> MAPLGYFLLLCSLKQALGSYPIWWSLAVGPQYSSLGSQPILCASIPGLVPKQLRFCRNYVEIMPSVAEGIKIGIQECQHQFRGRRWNCTTVHDSLAIFGPVLDKATRESAFVHAIASAGVAFAVTRSCAEGTAAICGCSSRHQGSPGKGWKWGGCSEDIEFGGMVSREFADARENRPDARSAMNRHNNEAGRQAIASHMHLKCKCHGLSGSCEVKTCWWSQPDFRAIGDFLKDKYDSASEMVVEKHRESRGWVETLRPRYTYFKVPTERDLVYYEASPNFCEPNPETGSFGTRDRTCNVSSHGIDGCDLLCCGRGHNARAERRREKCRCVFHWCCYVSCQECTRVYDVHTCK;> MAGAIIENMSTKKLCIVGGILLVFQIIAFLVGGLIAPGPTTAVSYMSVKCVDARKNHHKTKWFVPWGPNHCDKIRDIEEAIPREIEANDIVFSVHIPLPHMEMSPWFQFMLFILQLDIAFKLNNQIRENAEVSMDVSLAYRDDAFAEWTEMAHERVPRKLKCTFTSPKTPEHEGRYYECDVLPFMEIGSVAHKFYLLNIRLPVNEKKKINVGIGEIKDIRLVGIHQNGGFTKVWFAMKTFLTPSIFIIMVWYWRRITMMSRPPVLLEKVIFALGISMTFINIPVEWFSIGFDWTWMLLFGDIRQGIFYAMLLSFWIIFCGEHMMDQHERNHIAGYWKQVGPIAVGSFCLFIFDMCERGVQLTNPFYSIWTTDIGTELAMAFIIVAGICLCLYFLFLCFMVFQVFRNISGKQSSLPAMSKVRRLHYEGLIFRFKFLMLITLACAAMTVIFFIVSQVTEGHWKWGGVTVQVNSAFFTGIYGMWNLYVFALMFLYAPSHKNYGEDQSNGDLGVHSGEELQLTTTITHVDGPTEIYKLTRKEAQE

Wntless (WLS), an evolutionarily conserved multi-pass transmembrane protein, is essential for secretion of Wnt proteins. WLS has been found to directly interact with Wnts throughout the secretory route initiated from ER, then Golgi, secretory vesicles and finally cell membrane. Wnt-triggered signaling pathways control many crucial life events, whereas aberrant Wnt signaling is tightly associated with many human diseases including cancers. The transmembrane domain of WLS bears a GPCR fold, with a conserved core cavity and a lateral opening.

Here, we report a cryo-EM structure of wild type (WT) human WLS in complex with Wnt3a at 2.2 Å resolution. The built model comprises 496 residues of 541-residue WLS and 334 residues of Wnt3a after cleavage of signal peptide. In the overall structure, Wnt3a perches on the luminal side of WLS with several β-hairpin and loop regions (Hairpin-1, Hairpin-2 and W-loop) interacting with WLS extensively and generate three major interfaces. WLS looks like a grasping right hand that seizes one finger (Hairpin-1) of Wnt3a bearing the conserved palmitoleoylated Ser209, which is reported to be essential for Wnt secretion and interaction with Frizzled receptors on cell membrane. Wnt3a pinches WLS with another two fingers (Hairpin-2 and W-loop) at the luminal region of WLS. Wnt3a is palmitoleoylated with density for PAM clearly resolved, and the modification was confirmed by mass spectrometry. Intriguingly, we found in the TM domain of WLS there is a large hydrophobic cavity and a lateral opening between TM6 and TM7 that exposes the cavity to membrane environment. This cavity accommodates the extruding Hairpin-1 of Wnt3a, and one POPC molecule, clearly identified in the EM map. At Interface 2, Wnt3a Hairpin-2, containing Trp333 and stabilized by the disulfide bond formed between Cys334 and Cys335, extensively interacts with residues in a hydrophobic pocket at the distal region of WLS luminal domain. At Interface 3, Trp150 on Wnt3a W-loop forms hydrophobic interactions with Met101, Met103, and Phe107 in the loop between β-strand 2 (β2) and β-strand 3 (β3) of WLS luminal domain.>MNYPVNPDLMPALMAVFQHVRTRIQSELDCQRLDLTPPDVHVLKLIDEQRGLNLQDLGRQMCRDKALITRKIRELEGRNLVRRERNPSDQRSFQLFLTDEGLAIHQHAEAIMSRVHDELFAPLTPVEQATLV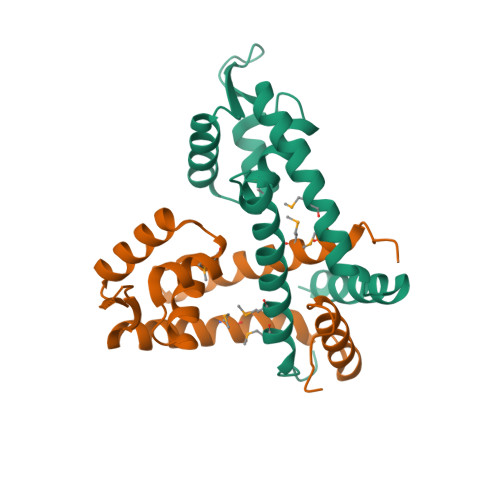HLLDQCLAAQPLEDI[8x]>APPRKVLIISAGASHSVALLSGDIVCSWGRGEDGQLGHGDAEDRPSPTQLSALDGHQIVSVTCGADHTVAYSQSGMEVYSWGWGDFGRLGHGNSSDLFTPLPIKALHGIRIKQIACGDSHCLAVTMEGEVQSWGRNQNGQLGLGDTEDSLVPQKIQAFEGIRIKMVAAGAEHTAAVTEDGDLYGWGWG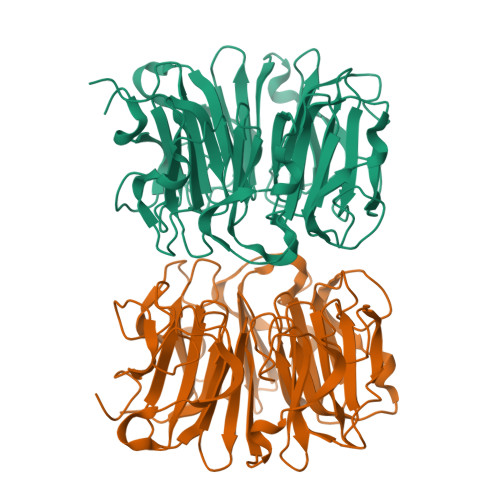RYGNLGLGDRTDRLVPERVTSTGGEKMSMVACGWRHTISVSYSGALYTYGWSKYGQLGHGDLEDHLIPHKLEALSNSFISQISGGFRHTMALTSDGKLYGWGWNKFGQVGVGNNLDQCSPVQVRFPDDQKVVQVSCGWRHTLAVTERNNVFAWGRGTNGQLGIGESVDRNFPKIIEALSVDG[4x]>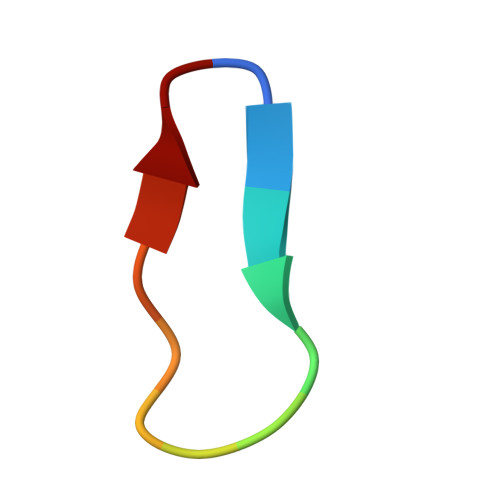 CWTTRMSPPMQIP> MTLEKFVDALPIPDTLKPVQQSKEKTYYEVTMEECTHQLHRDLPPTRLWGYNGLFPGPTIEVKRNENVYVKWMNNLPSTHFLPIDHTIHHSDSQHEEPEVKTVVHLHGGVTPDDSDGYPEAWFSKDFEQTGPYFKREVYHYPNQQRGAILWYHDHAMALTRLNVYAGLVGAYIIHDPKEKRLKLPSDEYDVPLLITDRTINEDGSLFYPSAPENPSPSLPNPSIVPAFCGETILVNGKVWPYLEVEPRKYRFRVINASNTRTYNLSLDNGGDFIQIGSDGGLLPRSVKLNSFSLAPAERYDIIIDFTAYEGESIILA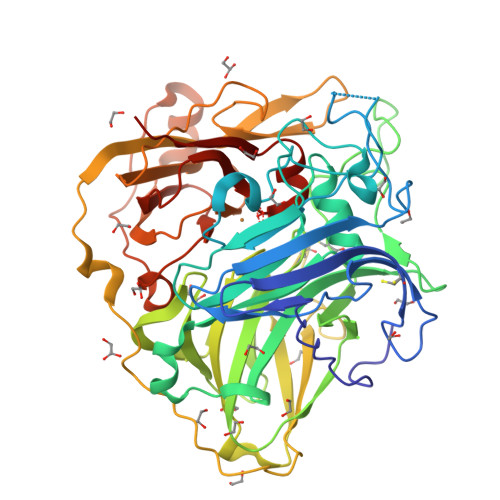NSAGCGGDVNPETDANIMQFRVTKPLAQKDESRKPKYLASYPSVQHERIQNIRTLKLAGTQDEYGRPVLLLNNKRWHDPVTETPKVGTTEIWSIINPTRGTHPIHLHLVSFRVLDRRPFDIARYQESGELSYTGPAVPPPPSEKGWKDTIQAHAGEVLRIAATFGPYSGRYVWHCHILEHLDYDMMRPMDITDPHK[4-amino-2-(tert-butylamino)-1,3-thiazol-5-yl](phenyl)methanone | C14 H17 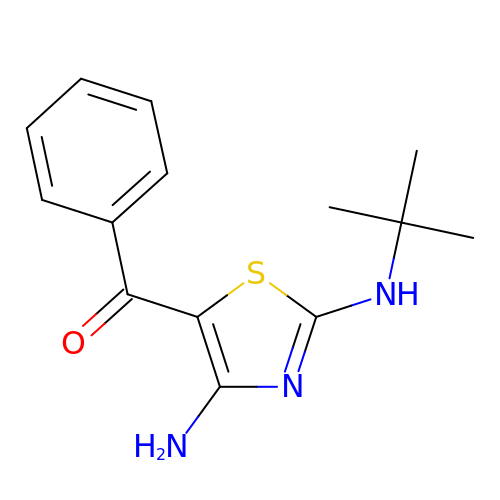N3 O S | KEHNGAHNKVLUSC-UHFFFAOYSA-N2,2-dimethylpropanamide | 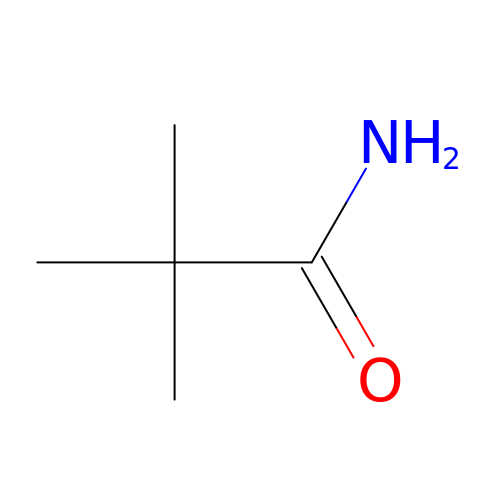C5 H11 N O | XIPFMBOWZXULIA-UHFFFAOYSA-N>[2x]MKIAVMTDSTSYLSQDLIDKYNIQIAPLSVTFDDGKNFTESNEIAIEEFYNKMASSQTIPTTSQPAIGEWITKYE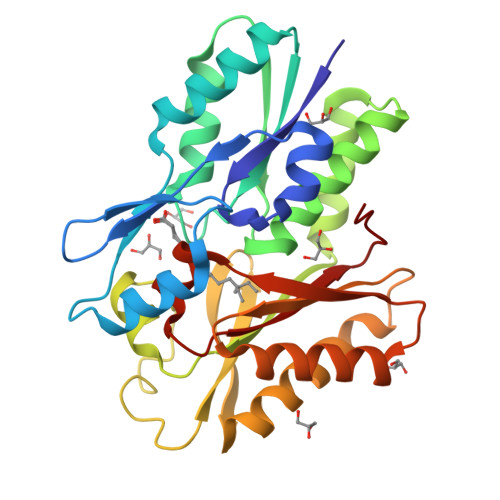MLRDQGYTDIIVICLSSGISGSYQSSYQAGEMVEGVNVHAFDSKLAAMIEGCYVLRAIEMVEEGYEPQQIIDDLTNMREHTGAYLIVDDLKNLQKSGRITGAQAWVGTLLKMKPVLKFEDGKIIPEEKVRTKKRAIQTLEKKVLDIVKDFEEVTLFVINGDHFEDGQALYKKLQDDCPSAYQVAYSEFGPVVAAHLGSGGLGLGYVGRKIRLT(E,7R)-7-[(1R,3aS,4E,7aR)-7a-methyl-4-[2-[(3R,5R)-4-methylidene-3,5-bis(oxidanyl)cyclohexylidene]ethylidene]-2,3,3a,5,6,7-hexahydro-1H-inden-1-yl]oct-2-en-4-one 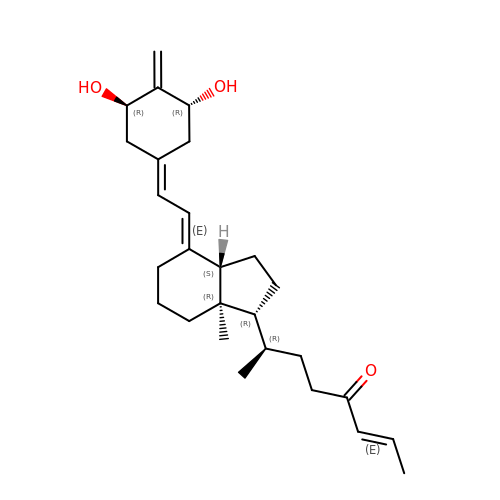| C27 H40 O3 | VGMKRRGYTONKLW-FOWSJJJVSA-N In particular, RORγt, whose activity is required for the proliferation and functionality of immune Th17 cells, is the subject of intense investigation to modulate its activity to achieve clinical benefit. NRs are characterized by the ability to bind small ligands at a highly conserved hydrophobic orthosteric-binding pocket located within the protein's ligand-binding domain (LBD). Helix 12 (H12, also called activation function-2, AF-2) can adopt distinct conformations in response to ligand binding, regulating the interaction of the LBD with cofactor proteins with resulting changes in gene transcription at a particular locus. Here we characterize the mode of action of these inhibitors to guide an optimization program and surprisingly find a novel binding mode, thereby identifying the first allosteric-binding pocket for a highly potent, cellular active small NR ligand.

To elucidate the molecular basis of RORγt modulation by MRL-871, we performed co-crystallization studies with an equimolar complex of RORγt-LBD and MRL-871. Co-crystals grew in two different space groups. Crystals in space group P6122 had unit cell dimensions of a=b=108.5, c=104.7 Å, diffracted to 2.2 Å resolution and also contain one molecule per asymmetric unit. The overall structures from both sets were identical in all the features and the ligand conformation. MRL-871 binds instead to a previously unidentified allosteric pocket in the RORγt LBD, located distal to the classical binding site (orange). Crystal structure analysis shows that this allosteric pocket, absent in the classical NR-folding motif, is formed by helices 4, 5, 11 and the reoriented flexible H12. Hydrogen-bonding interactions exist between the molecule's carboxylic acid group and the side chain of RORγt residue Q329 as well as the main-chain amide hydrogen atoms of residues A497 and F498. The unique conformation induced by the binding of MRL-871 prevents interaction with cofactor peptides, which typically bind RORγt through a conserved LXXLL motif, at the AF-2. MRL-871, however, effectively antagonizes the RORγt coactivator peptide recruitment interaction, independent of cholesterol concentration. In contrast, the inverse agonist T0901317 competes for the same binding site as cholesterol, resulting in a competitive displacement and a cholesterol concentration-dependent increase of the IC50 value for T0901317; that is, RORγt binding and inhibition by T0901317 becomes less potent in the presence of agonistic ligands. Together, these data demonstrate that the allosteric inhibition of coactivator binding to RORγt by MRL-871 is both potent and independent of orthosteric site occupancy.

> LTEIEHLVQSVCKSYRETCQLRLEDLLRQRSNIFSREEVTGYQRKSMWEMWERCAHHLTEAIQYVVEFAKRLSGFMELCQNDQIVLLKAGAMEVVLVRMCRAYNADNRTVFFEGKYGGMELFRALGCSELISSIFDFSHSLSALHFSEDEIALYTALVLINAHRPGLQEKRKVEQLQYNLELAFHHHLHKTHRQSILAKLPPKGKLRSLCSQHVERLQIFQHLHPIVVQAAFPPLYKELFS5-methyl-1-phenyl-1,2,3-triazole-4-carboxylic 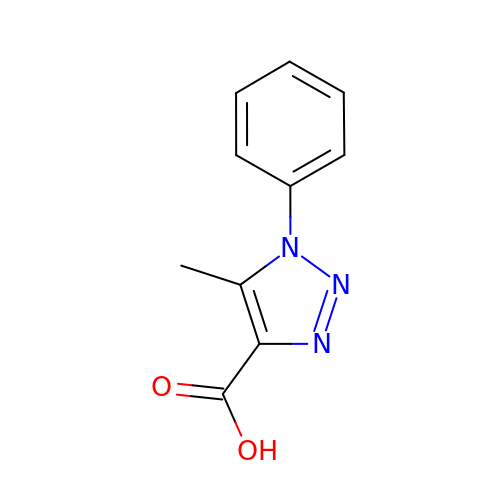acid | C10 H9 N3 O2 | RRHCZOBPABYIJZ-UHFFFAOYSA-N N-[(AMINOOXY)CARBONYL]-N-PHENYLAMINE | 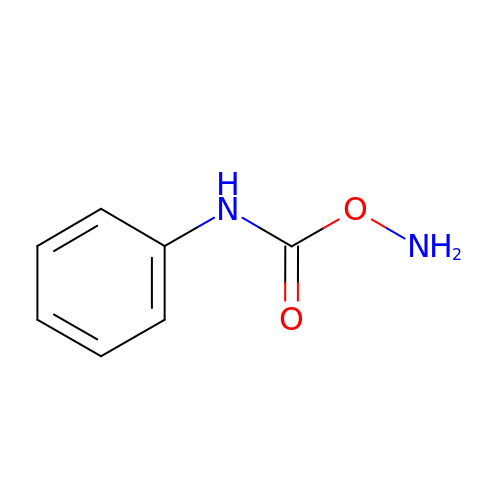C7 H8 N2 O2 | YQHOHPOCZUAUKP-UHFFFAOYSA-N> MLKKLKNFILFSSIFSPIAFAISCSNTGVVKQEDVSVSQGQWDKSITFGVSEAWLNKKKGGEKVNKEVINTFLENFKKEFNKLKNANDKTKNFDDVDFKVTPIQDFTVLLNNLSTDNPELDFGINASGKLVEFLKNNPGIITPALETTTNSFVFDKEKDKFYVDGTDSDPLVKIAKEINKIFVETPYASWTDENHKWNGNVYQSVYDPTVQANFYRGMIWIKGNDETLAKIKKAWNDKDWNTFRNFGILHGKDNSSSKFKLEETILKNHFQNKFTTLNEDRSAHPNAYKQKSADTLGTLDDFHIAFSEEGSFAWTHNKSATKPFETKANEKMEALIVTNPIPYDVGVFRKSVNQLEQN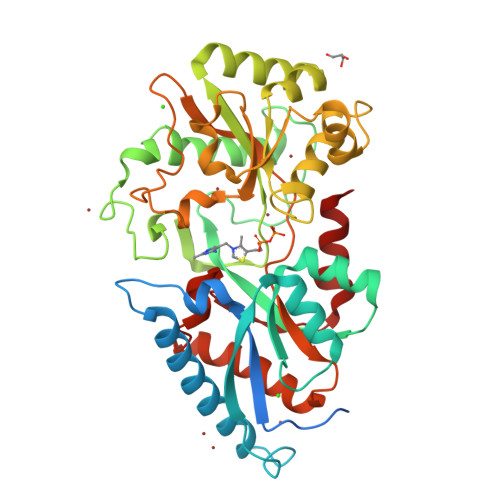LIVQTFINLAKNKQDTYGPLLGYNGYKKIDNFQKEIVEVYEKAIK> TGGCDVSARDVTVTLPDYPGSVPIPLTVYCAKSQNLGYYLSGTTADAGNSIFTNTASFSPAQGVGVQLTRNGTIIPANNTVSLGAVGTSAVSLGLTANYARTGGQVTAGN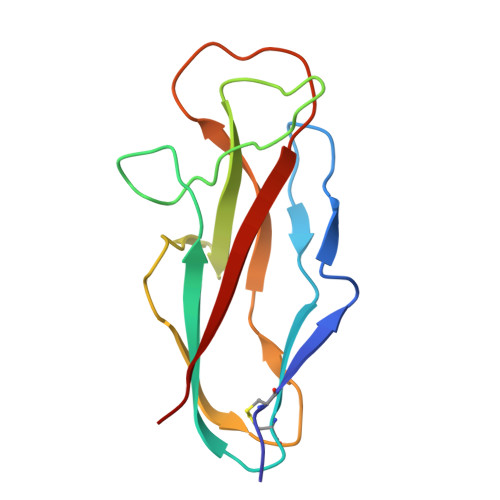VQSIIGVTFVYQ> SNANREDRNVLRMKERERRNQEIQQGEDAFPPSSPLFAEPYKVTSKEDKLSSRIQSMLGNYDEMK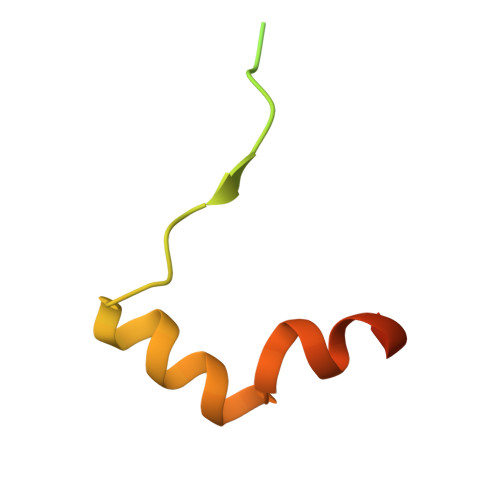DFIGDRSIPK> MQFLQNIPPYLFFTGKGGVGKTSISCATAIRLAEQGKRVLLVSTDPASNVGQVFSQTIGNTIQAIASVPGLSALEIDPQAAAQQYRARIVDPIKGVLPDDVVSSINEQLSGACTTEIAAFDEFTGLLTDASLLTRFDHIIFDTAPTGHTIRLLQLPGAWSSFIDSNPEGASCLGPMAGLEKQREQYAYAVEALSDPKRTRLVLVARLQKSTLQEVARTHLELAAIGLKNQYLVINGVLPKTEAANDTLAAAIWEREQEALANLPADLAGLPTDTLFLQPVNMVGVSALSRLLSTQPVASPSSDEYLQQRPDIPSLSALVDDIARNEHGLIMLMGKGGVGKTTMAAAIAVRLADMGFDVHLTTSDPAAHLSMTLNGSLNNLQVSRIDPHEETERYRQHVLETKGKELDEAGKRLLEEDLRSPCTEEIAVFQAFSRVIREAGKRFVVMDTAPTGHTLLLLDATGAYH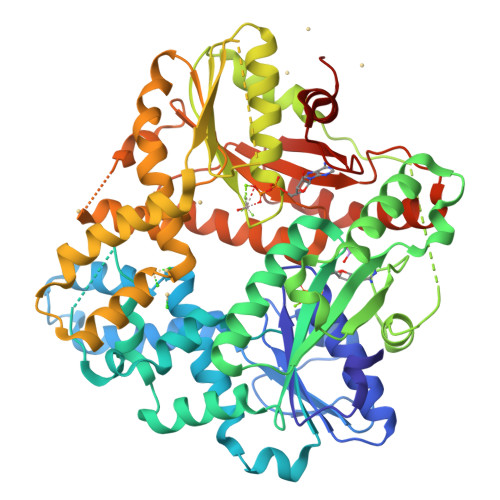REIAKKMGEKGHFTTPMMLLQDPERTKVLLVTLPETTPVLEAANLQADLERAGIHPWGWIINNSLSIADTRSPLLRMRAQQELPQIESVKRQHASRVALVPVLASEPTGIDKLKQLAGHHHHHH>[2x]GAMATAMYLEHYLDSIENLPSELQRNFQLMRELDQRTEDKKA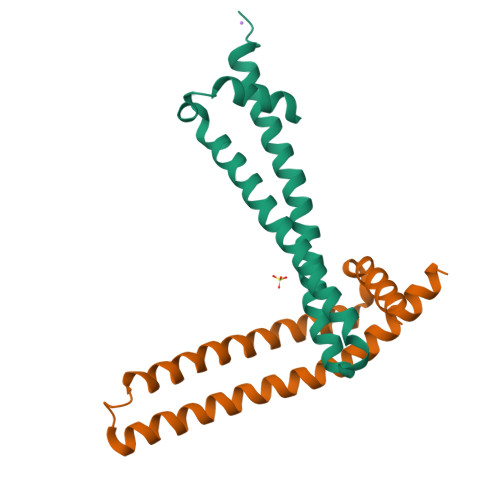EIDILAAEYISTVKTLSPDQRVERLQKIQNAYSKCKEYSDDKVQLAMQTYEMVDKHIRRLDADLA> GSQKHMKKGRTLMTFVSVTGNPTREESDTITKLWQTSLWNNHIQAERYMVDDNRAIFLFKDG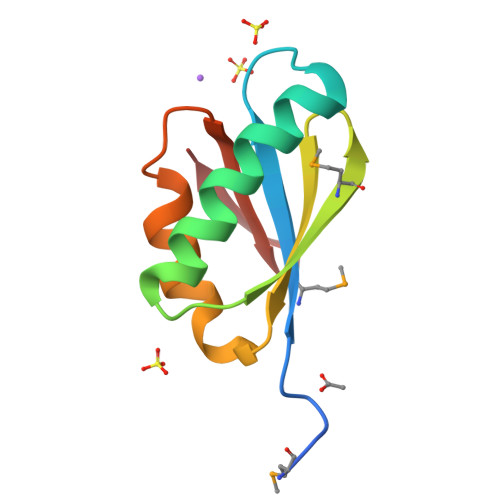TQAWDAKDFLIEQERCKGVTIENKEYPG>[4x]MAALRQPQVAELLAEARRAFREEFGAEPELAVSAPGRVNLIGEHTDYNQGLVLPMALELMTVLVGSPRKDGLVSLLTTSEGADEPQRL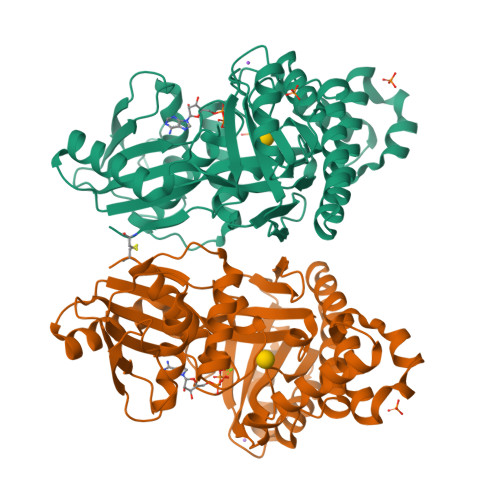QFPLPTAQRSLEPGTPRWANYVKGVIQYYPAAPLPGFSAVVVSSVPLGGGLSSSASLEVATYTFLQQLCPDSGTIAARAQVCQQAEHSFAGMPCGIMDQFISLMGQKGHALLIDCRSLETSLVPLSDPKLAVLITNSNVRHSLASSEYPVRRRQCEEVARALGAASLREVQLEELEAARDLVSKEGFRRARHVVGEIRRTAQAAAALRRGDYRAFGRLMVESHRSLRDDYEVSCPELDQLVEAALAVPGVYGSRMTGGGFGGCTVTLLEASAAPHAMRHIQEHYGGTATFYLSQAADGAKVLCL ethyl (2S)-oxiran-2-ylacetate | C6 H10 O3 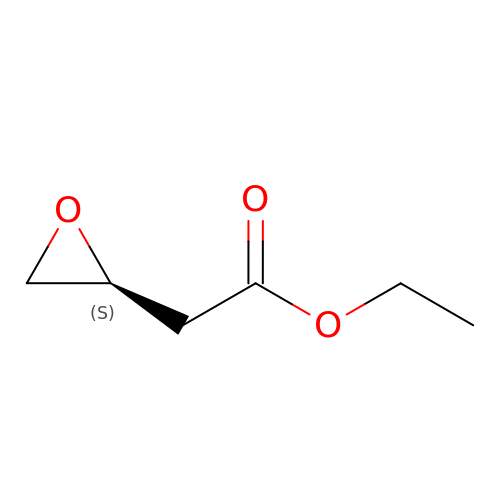| WHUSTVAXKRFVPD-YFKPBYRVSA-N2-[({4-[(4-tert-butylphenyl)methyl]piperazin-1-yl}sulfonyl)amino]-5-[(2-phenylethyl)sulfanyl]benzoic acid | C30 H37 N3 O4 S2 | 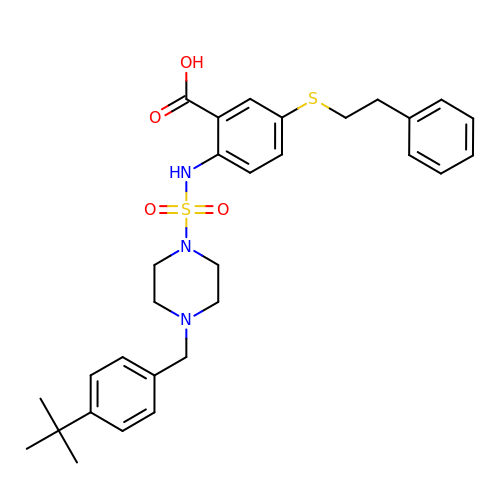WIWNZUYJVZDDEH-UHFFFAOYSA-N[5-(4-azanyl-2-oxidanylidene-pyrimidin-1-yl)-3-oxidanyl-furan-2-yl]methyl 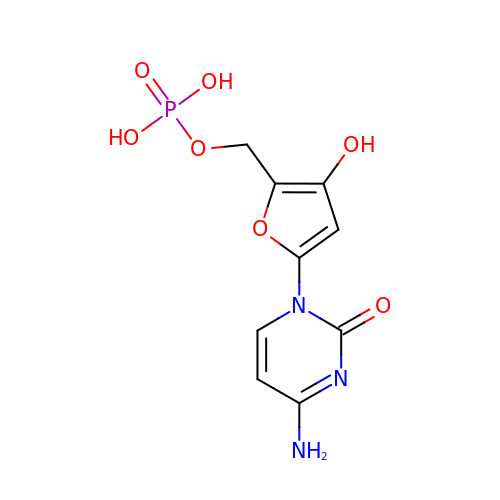dihydrogen phosphate | C9 H10 N3 O7 P | ZPERLPSVNPNRDZ-UHFFFAOYSA-N Adenylate kinase (AK) is a phosphotransferase enzyme catalyzing interconversion between ATP/AMP and two ADPs and is inhibited by P1,P5-di(adenosine 5′)-pentaphosphate (Ap5A), which mimics two adenylate substrates. Structural studies have revealed three characteristic AK domains, namely, the CORE, AMPbind, and LID domains. In the present study, a structural comparison of AKp and AKm revealed suboptimal hydrophobic packing in the CORE domain of the psychrophilic homologue, where a polar side chain makes contact with hydrophobic neighboring residues. We also determined the crystal structures of two AK mutants, which showed the largest thermal stability transition compared to wild-type (WT) AKs.

One such position was residue 26, located in the loop connecting α1 and β2. This residue belongs to the central CORE domain (residues 1–30, 60–126, and 164–217), which are known to be important for the overall structural stability of AKs. Mesophilic AKm contains Ile26 at this position, and its side chain is in close proximity (<5 Å) to other hydrophobic CORE residues, including Met1, Leu3, Val21, Tyr24, and Leu82. Notably, a thermally stable AK homologue from a thermophilic bacterium Geobacillus stearothermophilus also has an Ile residue at this position,26 supporting that Ile26 is important for optimal hydrophobic CORE packing and thermal stabilization of AKm. Mutation of Ile26 in the mesophilic AKm to Thr (as found in psychrophilic AKp) resulted in a 7.0 °C reduction in Tm. The I26T mutation in AKm significantly reduced catalytic activities at high temperatures (55 and 65 °C), whereas the activities at low temperatures (5 °C to 45 °C) were similar between the WT and mutant enzymes. In contrast, in the crystal structure of the AKm I26T mutant, the polar side chain of the mutated Thr26 residue cannot have these hydrophobic contacts with other non-polar residues in the CORE domain. Consistently, the I26T substitution reduced the apolar buried surface area in AKm.

> MNLVLMGLPGAGKGTQGERIVEDYGTPHISTGDMFRAAMKEETPLGLEAKSYIDKGELVPDEVTIGIVKERLGKDDCERGFLLDGFPRTVAQAEALEEILEEYGKPIDYVINIEVDKDVLMERLTGRRICSVCGTTYHLVFNPPKTPGICDKDGGELYQRADDNEETVSKRLEVNMKQTQPLLDFYSEKGYLANVNGQQDIQDVYADVKDLLGGLKK>MENDMKSLSAAAQACVKKMRDAKVNEACIRTFIAQHVMVSKGETGSIPDSAIMPVDSLDALDSLTIECDNAVLQSTVVLKLNGGLGTGMGLCDAKTLLEVKDGKTFLDFTALQVQYLRQHCSEHLRFMLMDSFNTSASTKSFLKARYPWLYQVFDSEVELMQNQVPKILQDTLEPAAWAENPAYEWAPPGHGDIYTALYGSGKLQELVEQGYRYMFVSNGDNLGATIDKRVLAYMEKEKIDFLMEVCRRTESDKKGGHLARQTVYVKGKDGQPDAEKRVLLLRESAQCPKADMESFQDINKYSFFNTNNLWIRLPVLLETMQEHGGTLPLPVIRNEKTVDSSNSASPKVYQLETAMGAAIAMFESASAIVVPRSRFAPVKTCADLLALRSDAYVVTDDFRLWLDDRCHGHPPVVDLDSAHYKMMNGFEKLVQHGVPSLVECKRVTVKGLVQFGAGNVLTGTVTIENTDSA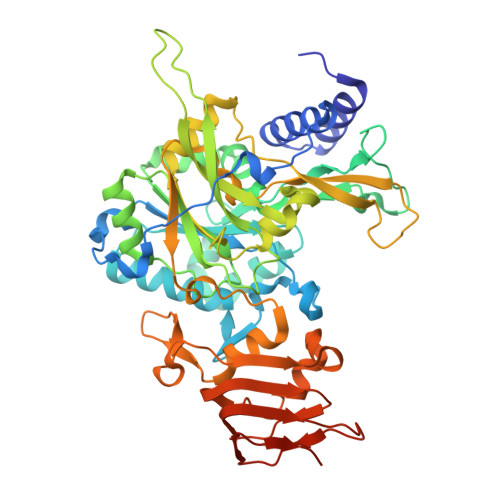SAFVIPDGAKLNDTTASPQQSTNKMRPLEHHHHHH[2x]>MQVLPPSSTGGPSRLFIMRPVATTLLMVAILLAGIIGYRALPVSALPEVDYPTIQVVTLYPGASPDVMTSAVTAPLERQF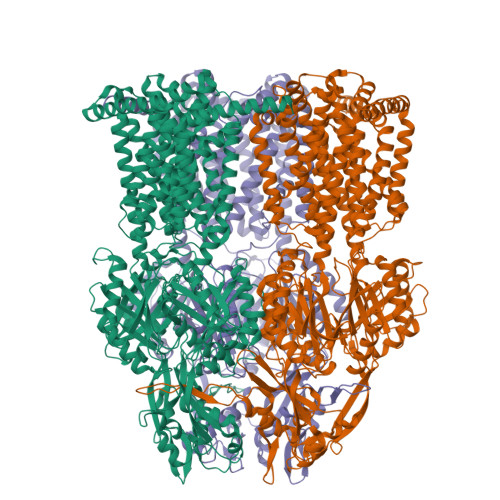GQMSGLKQMSSQSSGGASVITLQFQLTLPLDVAEQEVQAAINAATNLLPSDLPNPPVYSKVNPADPPIMTLAVTSTAMPMTQVEDMVETRVAQKISQISGVGLVTLSGGQRPAVRVKLNAQAIAALGLTSETVRTAITGANVNSAKGSLDGPSRAVTLSANDQMQSAEEYRQLIIAYQNGAPIRLGDVATVEQGAENSWLGAWANKEQAIVMNVQRQPGANIISTADSIRQMLPQLTESLPKSVKVTVLSDRTTNIRASVDDTQFELMMAIALVVMIIYLFLRNIPATIIPGVAVPLSLIGTFAVMVFLDFSINNLTLMALTIATGFVVDDAIVVIENISRYIEKGEKPLAAALKGAGEIGFTIISLTFSLIAVLIPLLFMGDIVGRLFREFAITLAVAILISAVVSLTLTPMMCARMLSQESLRKQNRFSRASEKMFDRIIAAYGRGLAKVLNHPWLTLSVALSTLLLSVLLWVFIPKGFFPVQDNGIIQGTLQAPQSSSFANMAQRQRQVADVILQDPAVQSLTSFVGVDGTNPSLNSARLQINLKPLDERDDRVQKVIARLQTAVDKVPGVDLFLQPTQDLTIDTQVSRTQYQFTLQATSLDALSTWVPQLMEKLQQLPQLSDVSSDWQDKGLVAYVNVDRDSASRLGISMADVDNALYNAFGQRLISTIYTQANQYRVVLEHNTENTPGLAALDTIRLTSSDGGVVPLSSIAKIEQRFAPLSINHLDQFPVTTISFNVPDNYSLGDAVQAIMDTEKTLNLPVDITTQFQGSTLAFQSALGSTVWLIVAAVVAMYIVLGILYESFIHPITILSTLPTAGVGALLALLIAGSELDVIAIIGIILLIGIVKKNAIMMIDFALAAEREQGMSPREAIYQACLLRFRPILMTTLAALLGALPLMLSTGVGAELRRPLGIGMVGGLIVSQVLTLFTTPVIYLLFDRLALWTKSRFARHEEEA[3x]N-(hydroxyacetyl)-beta-D-glucopyranosylamine | C8 H15 N O7 | 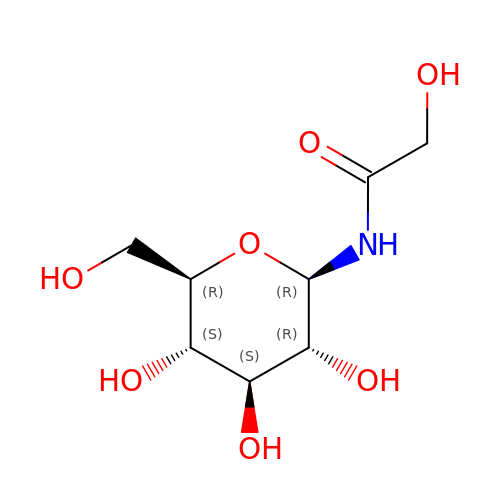DIGPTJYOVRRBRM-RHROMQPHSA-N(3S,6S)-3,6-bis(4-hydroxybenzyl)piperazine-2,5-dione | C18 H18 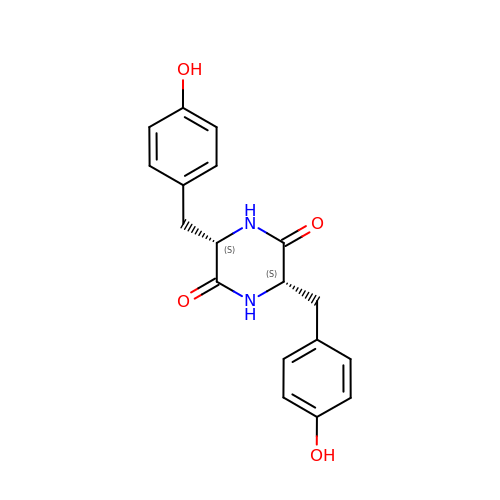N2 O4 | NGPCLOGFGKJCBP-HOTGVXAUSA-N>[4x]KTTYERTFVKKDAETKEVLEGAGFKISNSDGKFLKLTDKDGQSVSIGEGFIDVLANNYRLTWVAESDATVFTSDKSGKFGLNGFADNTTTYTAVETNVPDGYDAAANTDFKADNSSSDILDAPSGILPLEHHHHHH

As the first reported host of “non-pathogenic-derived” pili, Lactobacillus rhamnosus GG is a gut-adapted commensal lactic acid bacterium (LAB) and one of many clinically investigated probiotic strains for human use in the prevention and treatment of certain gastric ailments. As with other Gram-positive bacteria, sortase-dependent piliation in L. rhamnosus GG (called SpaCBA) is assembled from the ~30 kDa SpaA (backbone), ~20 kDa SpaB (basal), and ~90 kDa SpaC (tip-located) pilins. Two immunoglobulin (Ig)-like subdomains comprise GG-SpaA, each having the conserved residues of a canonical E-box motif and internal isopeptide bonds formed between either lysine and asparagine or lysine and aspartate residues. Our findings show that the GG-SpaA structure has certain features in common with other pathogen-derived pilin-proteins, such as the Ig-like CnaB-type folds and the presence of internal isopeptide bonds6940.

As an alternative, GG-SpaA protein was fragmented by limited proteolysis as had been done previously for other backbone pilins. This produced a 15 kDa-sized fragment that can be crystallized in two different forms. Intriguingly, six metal ions are associated with the C-domain when the structure was solved using orthorhombic crystals. Mainly owing to the crystals having been grown in the presence of 20 mM zinc sulphate, these metal ions were modeled putatively as zinc. Here, these metal ions can be seen at the surface between the molecules in the asymmetric unit stabilizing molecular packing in the crystal. Metal ions are primarily coordinated by aspartates, but glutamate, lysine, and water from asymmetric and symmetric molecules also seem to participate. Among known categories of zinc-binding sites in proteins, the metal ion coordination environment in GG-SpaA can be classified as an “interface type”, based on the incomplete coordination spheres, weak electron densities for the coordinated water molecules, and the location of the metal sites. Refined models for the tetragonal and orthorhombic crystals (residues 176–298) gave Rwork/Rfree values of 13.9%/15.8% and 21.6%/24.9%, respectively. The structure of a 15 kDa fragment of GG-SpaA that had been generated by limited proteolysis is identical to that of the C-domain of full-length GG-SpaA (see preceding section for details).> GSMTGWTAADLPSFAQRTVVITGANSGLGAVTARELARRGATVIMAVRDTRKGEAAARTMAGQVEVRELDLQDLSSVRRFADGVSGADVLINNAGIMAVPYALTVDGFESQIGTNHLGHFALTNLLLPRLTDRVVTVSSMAHWPGRINLEDLNWRSRRYSPWLAYSQSKLA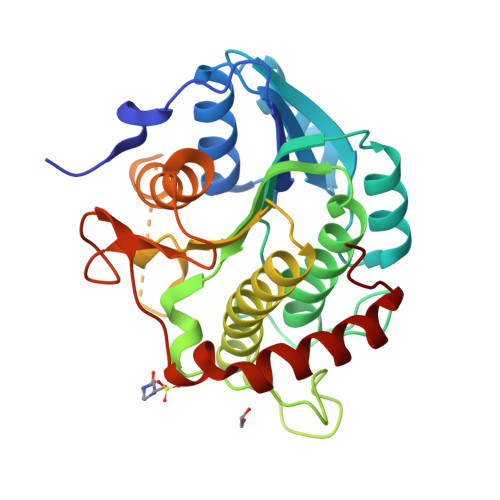NLLFTSELQRRLTAAGSPLRALAAHPGYSHTNLQGASGRKLGDALMSAATRVVATDADFGARQTLYAASQDLPGDSFVGPRFGYLGRTQPVGRSRRAKDAGMAAALWALSEQLTKTEFPL>LDSLLGQEKERFQVLPGRDKMLYVAAQNERDTLWARQVLARGDYDKNARVINENEENKRISIWLDTYYPQLAYYRIHFDEPRKPVFWLSRQRNTMSKKELEVLSQKLRALMPYADSVNITLMDDVTAAGQAEAGLKQQALPYSRRNHKGGVTFVIQGAL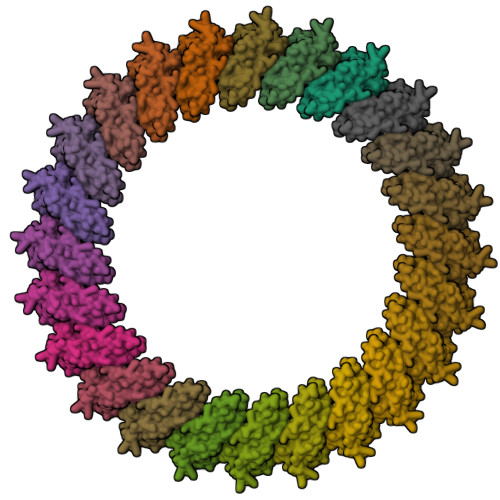DDVEILRARQFVDSYYRTWGGRYVQFAIELKD[24x]> GPGGDLHMDALLTKFNEDRSLQDENLSQPRTRVRIVDDNLYNKSNPFQLCYKKRDYGSQYYH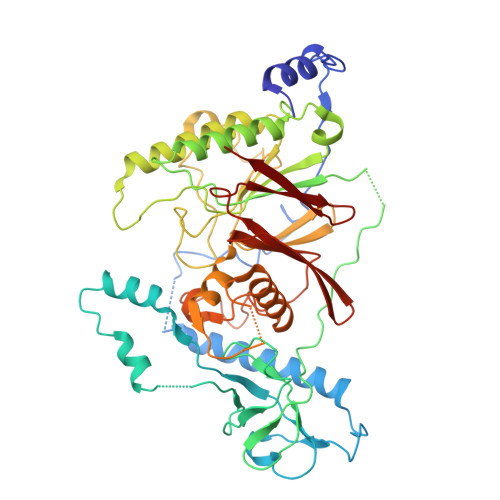IYQYRLKTFRERVLKECDKRWDAGFTLNGQLVLKKDKVLDIQGNQPCWCVGSIYCEMKYKPNVLDEVINDTYGAPDLTKSYTDKEGGSDEIMLEDESGRVLLVGDFIRSTPFITGVVVGILGMEAEAGTFQVLDICYPTPLPQNPFPAPIATCPTRGKIALVSGLNLNNTSPDRLLRLEILREFLMGRINNKIDDISLIGRLLICGNSVDFDIKSVNKDELMISLTEFSKFLHNILPSISVDIMPGTNDPSDKSLPQQPFHKSLFDKSLESYFNGSNKEILNLVTNPYEFSYNGVDVLAVSGKNINDICKYVIPSNDNGESENKVEEGESNDFKDDIEHRLDLMECTMKWQNIAPTAPDTLWCYPYTDKDPFVLDKWPHVYIVANQPYFGTRVVEIGGKNIKIISVPEFSSTGMIILLDLETLEAETVKIDI>[2x]GSHMIYSEFIMDYSKLKKFHGKIENAHKVEEGKNLSCGDEVTLYFLFDGDKIVDVKFEGHGCAISQASTNVMIEQIIGKTKQEALEMMKNAENMMLGKEFDE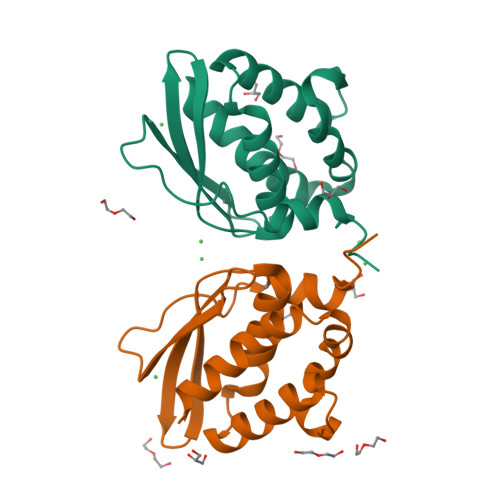NVLGPIINFYDVKNYPMRVKCFLLPWKTLEIALKNE> VTVGDQNGMGPSSGYVTRITNDAREDDMENNMKEVSSMIGNLRNMAIDMGNEIGSQNRQVDRIQQKAESNESRI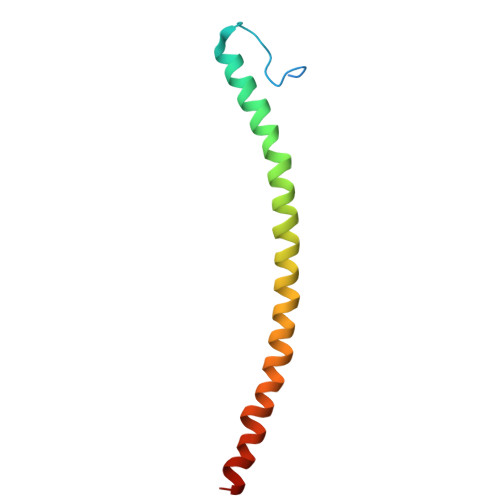DEANKKATKLLKN The C-terminus of the severe acute respiratory syndrome coronavirus 2 (SARS-CoV-2) protein E contains a PBM (PDZ-binding motif) targeting PDZ (PSD-95/Dlg/ZO-1) domains, which is identical to the PBM of SARS-CoV. Targeting multiple cellular PDZ (PSD-95/Dlg/ZO-1)-containing proteins through short linear PDZ-binding motifs (PBMs) is a common strategy used by viruses to facilitate their viral replication and dissemination to new hosts. PBMs are mainly located at the C-terminus of target proteins and interact directly with PDZ domains. We solved three crystal structures of complexes between human LNX2, MLLT4, and MPP5 PDZs and SARS-CoV-2 E PBM highlighting its binding preferences for several cellular targets.

MLLT4 is an adapter protein linking nectin to the actin cytoskeleton, essential for the formation of adherent junctions and the regulation of cell adhesion. The crystal structure of MLLT4-PDZ in complex with SARS-CoV-2-E-PBM peptide was solved at a resolution of 2.28 Å. The final refined model contains two PDZ domains per asymmetric unit that adopt a swapped dimer conformation with the PDZ folding comprising five β strands and two α helices. Two peptides are bound to each PDZ dimer. The swapped dimer comprises an intermolecular interaction between the two PDZ domains through the β1/β6 pair, and several pairs of inter-domain H-bonds between the fragments Lys 1014–Gly 1017 of each chain. The MLLT4-PDZ is found mainly monomeric in solution with a sedimentation coefficient of 1.4 S, suggesting that the swapped dimer is probably an artifact of crystallization. The E PBM binds to the PDZ in a conventional manner as an antiparallel extension of the β2 strand by inserting into a binding groove formed by the β2 strand, the α2 helix, and the “GLGF” motif. The C-terminal carboxylate of Val at position 0 of the PBM forms three hydrogen bonds with the amide protons of Met 1018, Gly 1019, and Leu 1020 of the “GLGF” loop of MLLT4-PDZ. In addition, the carbonyl and the amide group of Leu at position -2 interacts through a hydrogen bond with the proton amide and the carbonyl group of Ile 1022, respectively. A hydrogen bond is also formed between the carboxyl at the end of the side chain of Asp at position -3 of the PBM and the hydroxyl of Ser 1021 of the β2 strand.

>[2x]GRKEPEIITVTLKKQNGMGLSIVAAKGAGQDKLGIYVKSVVKGGAADVDGRLAAGDQLLSVDGRSLVGLSQERAAELMTRTSSVVTLEVAKQGAIYH;>NLNSSRVPDLLV[2x]> NNELSPVALRQMSCAAGTTQTACTDDNALAYYNTTKGGRFVLALL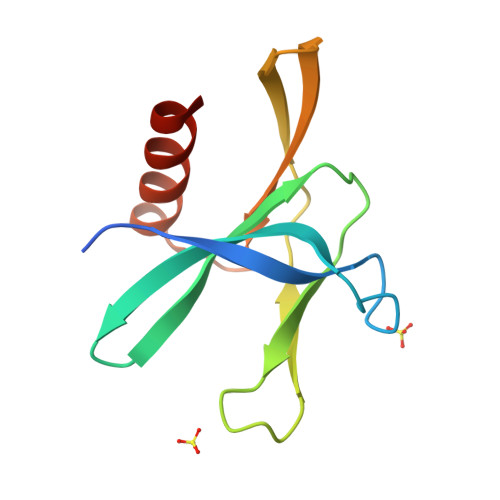SDLQDLKWARFPKSDGTGTIYTELEPPCRFVTDTPKGPKVKYLYFIKGLNNLNRGMVLGSLAATVRLQ>[2x]MGSKKLTVGSDSHRLSKSSFSSNKSSHSATKDQPIDTDDIDEDDESGHNIILNIISQLRPGCDLTRITLPTFILEKKSMLERVTNQLQFPEFLLQAHSEKDPLKRFLYVMKWYLAGWHIAPKAVKKPLNPVLGEYFTAYWDLPNKQQAYYISEQTSHHPPECAYFYMIPESSIRVDGVVIPKSRFLGNSSAAMMDGSTVLQFLDIKDGNGKPEKYVLTQ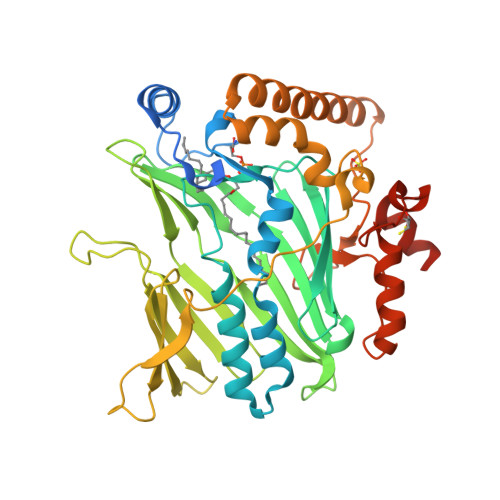PNVYVRGILFGKMRIELGDHMIIKSPNFQADIEFKTKGYVFGTYDAIEGTVKDYDGNAYYEISGKWNDVMYLKDLKQPRSSPKVFLDTHKESPLRPKVRPLSEQGEYESRKLWKKVTDALAVRNHPVATEEKFQIEDHQRQLAKKRIEDGVEFHPKLFRRSKPGEDLDYCIYKNIPVDEDPEKQIRSILQIAPILPGQQFTDKFFIPAFEKIKSQKKMIENEKQNPAKQ> MISYDNYVTILDEETLKAWIAKLEKAPVFAFATATDSLDNISANLVGLSFAIEPGVAAYIPVAHDYLDAPDQISRERALELLKPLLEDEKALKVGQNLKYDRGILANYGIELRGIAFDTMLESYILNSVAGRHDMDSLAERWLKHKTITFEEIAGKGKNQLTFNQIALEEAGRYAAEDADVTLQLHLKMWPDLQKHKGPLNVFENIEMPLVPVLSRIERNGVKIDPKVLHNHSEELTLRLAELEKKAHEIAGEEFNLSSTKQLQTILFEKQGIKPLKKTPGGAPSTSEEVLEELA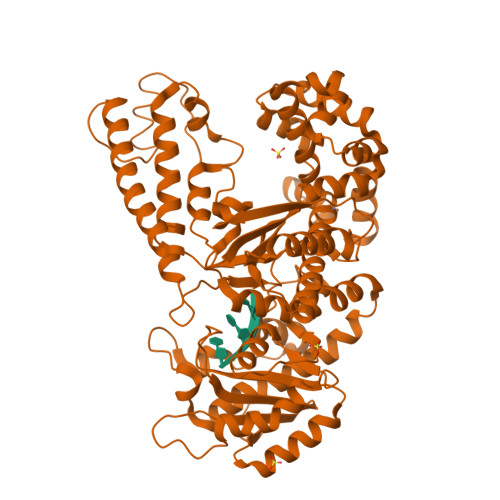LDYPLPKVILEYRGLAKLKSTYTDKLPLMINPKTGRVHTSYHQAVTATGRLSSTDPNLQNIPVRNEEGRRIRQAFIAPEDYVIVSADYSQIELRIMAHLSRDKGLLTAFAEGKDIHRATAAEVFGLPLETVTSEQRRSAKAINFGLIYGMSAFGLARQLNIPRKEAQKYMDLYFERYPGVLEYMERTRAQAKEQGYVETLDGRRLYLPDIKSSNGARRAAAERAAINAPMQGTAADIIKRAMIAVDAWLQAEQPRVRMIMQVHDELVFEVHKDDVDAVAKQIHQLMENCTRLDVPLLVEVGSGENWDQAH> GKSEISELRRTMQNLEIELQSQLSMKASLENSLEE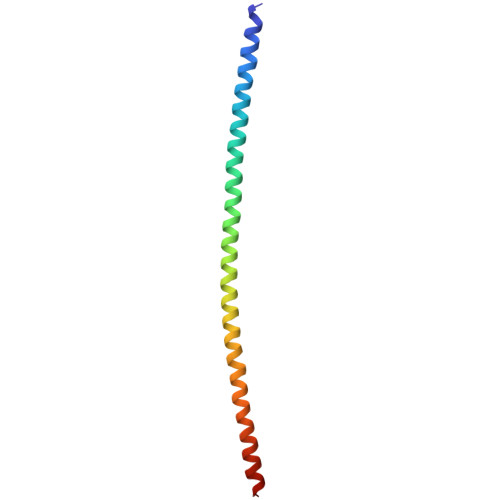TKGRYAMQLAQIQEMIGSVEEQLAQLRCEMEQQNQEYKILLDVKTRLEQEIATYRRLLEG>[2x]AQKSVKISDDISITQLSDKVYTYVSLAEIEGWGMVPSNGMIVINNHQAALLDTPINDAQTEMLVNWVTDSLHAKVTTFIPNHWHGDCIGGLGYLQRKGVQSYANQMTIDLAKE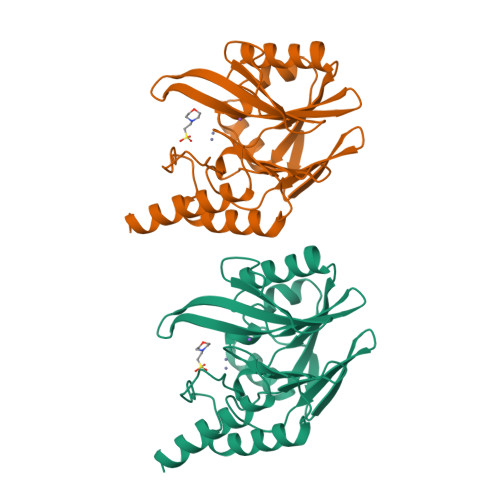KGLPVPEHGFTDSLTVSLDGMPLQCYYLGGGHATDNIVVWLPTENILFGGCMLKDNQTTSIGNISDADVTAWPKTLDKVKAKFPSARYVVPGHGNYGGTELIEHTKQIVNQYIESTSKP>[2x]GWKQQQIPQIKSNQENINTLKYKELIAGELMRITHKLLIQKLQQQQPANNNKQINEMDVESNELAEKKEVIIKIQEIAKDQQLYDTLSIQYQVDQ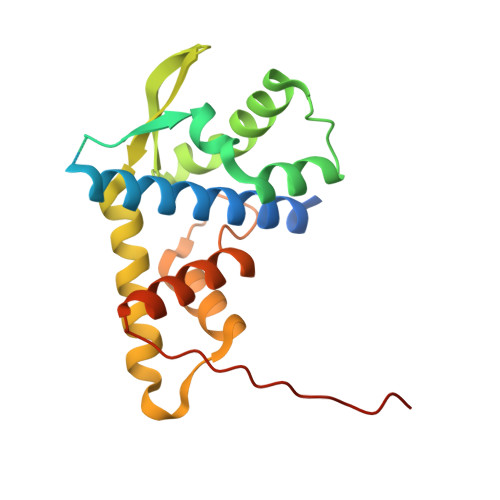KEQYYAKIAQSLEDFVSISALKMVSYIYPNISYQVSIGFFQNILDIATKTVKDRGALGCNYKYLKDKLTKALNLQQISYPLISESYISYLVHLFQDFNIIEIENEHKFYYKQAFQYDDS6,6'-{[5-(3-aminopropyl)benzene-1,3-diyl]diethane-2,1-diyl}bis(4-methylpyridin-2-amine) | C25 H33 N5 | 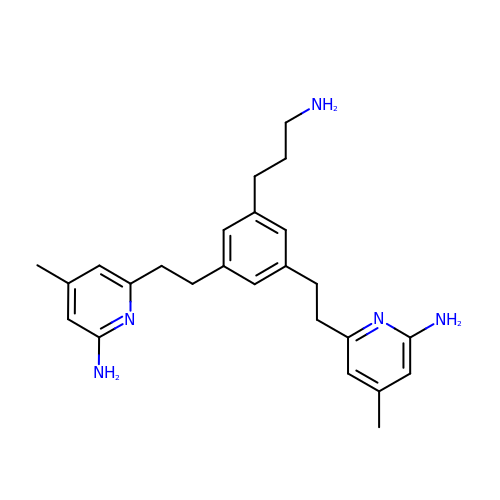TUMIYXWSFLIVFR-UHFFFAOYSA-N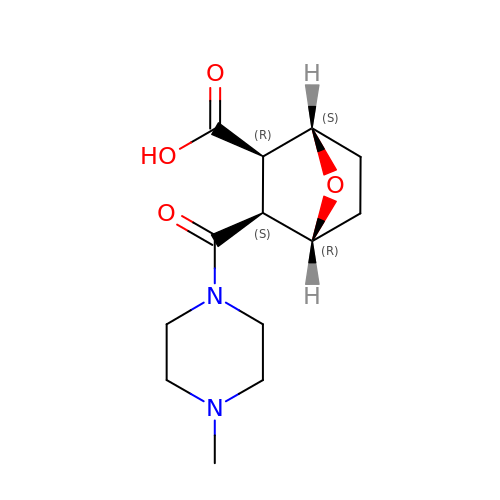(1S,2R,3S,4R)-3-(4-methylpiperazine-1-carbonyl)-7-oxabicyclo[2.2.1]heptane-2-carboxylic acid | C13 H20 N2 O4 | JUQMLSGOTNKJKI-YTWAJWBKSA-N>[2x]MPAGHEEFDIPFPSRVNPFHARAEDRHVAWMRAMGLITGDAAEATYRRWSPAKVGARWFYLAQGEDLDLGCDIFGWFFAYDDHFDGPTGTDPRQTAAFVNRTVAMLDPRADPTG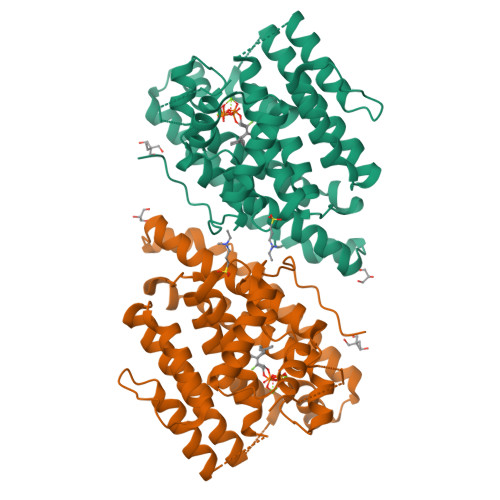EHPLNIAFHDLWQRESAPMSPLWQRRAVDHWTQYLTAHITEATNRTRHTSPTIADYLELRHRTGFMPPLLDLIERVWRAEIPAPVYTTPEVQTLLHTTNQNINIVNDVLSLEKEEAHGDPHNLVLVIQHERQSTRQQALATARRMIDEWTDTFIRTEPRLPALCGRLGIPLADRTSLYTAVEGMRAAIRGNYDWCAETNRYAVHRPTGTGRATTPW>MAHHHHHHMIREILKMGDP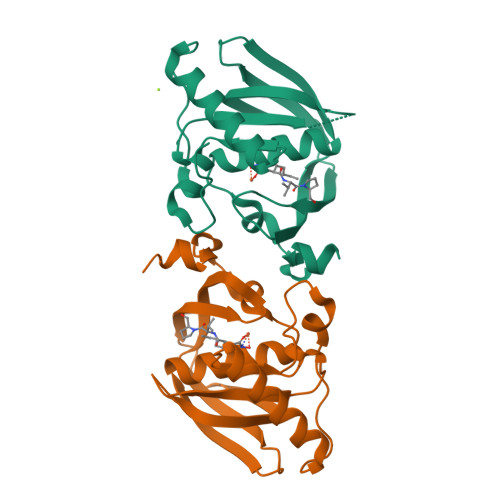RLLRIADPVDHFDTPELHELVKDMFETMHDANGAGLAAPQIGVNLQVVIFGFGHNERYPDAPPVPETVLINPTITPVSQDMEEGWEGCLSVPGLRGAVSRFSMIKYHGFDQYGKPIDRVAEGFHARVVQHECDHLIGKLYPMRINDFAKFGFTEVLFPDMDPNSDD[4x]> MHHHHHHKSTKILILGAGPAGFSAAKAALGKCDDITMINSEKYLPYYRPRLNEIIAKNKSIDDILIKKNDWYEKNNIKVITSEFATSIDPNNKLVTLKSGEKIKYEKLIIASGSIANKIKVPHADEI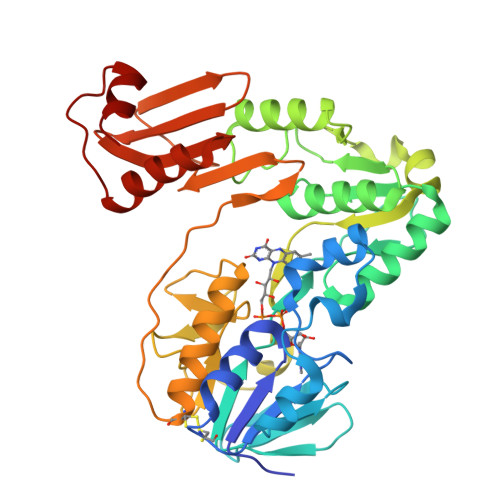FSLYSYDDALKIKDECKNKGKAFIIGGGILGIELAQAIIDSGTPASIGIILEYPLERQLDRDGGLFLKDKLDRLGIKIYTNSNFEEMGDLIRSSCVITAVGVKPNLDFIKDTEIASKRGILVNDHMETSIKDIYACGDVAEFYGKNPGLINIANKQGEVAGLNACGEDASYSEIIPSPILKVSGISIISCGDIENNKPSKVFRSTQEDKYIVCMLKENKIDAAAVIGDVSLGTKLKKAIDSSKSFDNISSLDAILNNL> GLVPRGSHMMEILRGSPALSAFRINKLLARFQAANLQVHNIYAEYVHFADLNAPLNDSEQAQLTRLLQYGPALSSHTPAGKLLLVTPRPGTISPWSSKATDIAHNCGLQQVDRLERGVAYYIEASTLTAEQWRQVAAELHDRMMETVFSSLTDAEKLFIHHQPAPVSSVDLLGEGRQALIDANLRLGLALAEDEIDYLQEAFTKLGRNPNDIELYMFAQANSEHCRHKIFNADWIIDGKPQPKSLFKMIKNTFETTPDYVLSAYKDNAAVMEGSAVGRYFADHNTGRYDFHQEPAHILMKVETHNHPTAISPWPGAATGSGGEIRDEGATGRGAKPKAGLVGFSVSNLRIPGFEQPWEEDFGKPERIVTALDIMTEGPLGGAAFNNEFGRPALTGYFRTYEEKVNSHNGEELRGYHKPIMLAGGIGNIRADHVQKGEIVVGAKLIVLGGPAMNIGLGGGAASSMASGQSDADLDFASVQRDNPEMERRCQEVIDRCWQLGDANPILFIHDVGAGGLSNAMPELVSDGGRGGKFELRDILSDEPGMSPLEIWCNESQERYVLAVAADQLPLFDELCKRERAPYAVIGDATEEQHLSLHDNHFDNQPIDLPLDVLLGKTPKMTRDVQTLKAKGDALNRADITIADAVKRVLHLPTVAEKTFLVTIGDRTVTGMVARDQMVGPWQVPVADCAVTTASLDSYYGEAMSIGERAPVALLDFAASARLAVGEALTNIAATQIGDIKRIKLSANWMAAAGHPGEDAGLYDAVKAVGEELCPQLGLTIPVGKDSMSMKTRWQEGNEQREMTSPLSLVISAFARVEDVRHTLTPQLSTEDNALLLIDLGKGHNALGATALAQVYRQLGDKPADVRDVAQLKGFYDAMQALVAARKLLAWHDRSDGGLLVTLAEMAFAGHCGVQVDIAALGDDHLAALFNEELGGVIQVRAEDRDAVEALLAQYGLADCVHYLGQALAGDRFVITANDQTVFSESRTTLRVWWAETTWQMQRLRDNPQCADQEHEAKANDTDPGLNVKLSFDINEDIAAPYIATGARPKVAVLREQGVNSHVEMAAAFHRAGFDAIDVHMSDLLGGRIGLGNFHALVACGGFSYGDVLGAGEGWAKSILFNHRVRDEFETFFHRPQTLALGVCNGCQMMSNLRELIPGSELWPRFVRNHSDRFEARFSLVEVTQSPSLLLQGMVGSQMPIAVSHGEGRVEVRDDAHLAALESKGLVALRYVDNFGKVTETYPANPNGSPNGITAVTTENGRVTIMMPHPERVFRTVANSWHPENWGEDSPWMRIFRNARKQLG

FGAR-AT encoded by the purL gene is a multidomain bi-functional enzyme that catalyzes the fourth step of the purine biosynthesis pathway. The FGAR-AT protein from Salmonella typhimurium (StPurL) has 1295 amino acid residues and is a single chain protein with three major domains. The C-terminal glutaminase domain produces an ammonia molecule that is consumed at the coupled active site present in the formylglycinamidine ribonucleotide (FGAM) synthetase domain where nitrogen is incorporated into an FGAR molecule converting it into FGAM. While the FGAM synthetase domain and glutaminase domain carry out the two enzymatic reactions within this bi-functional enzyme, the function of the N-terminal domain is not clearly understood.

The native crystals of StPurL protein were exposed to xenon gas and it was noticed that crystals derivatized for 5 min or longer at 40 bar, diffracted worse than 4.0 Å resolution. Moreover, solving the structure of StPurL protein crystals (StPurL-Xenon complex) which were pressurized for 4 min did not show any increase in the number of xenon atoms bound as compared to the crystals derivatized for 1 min therefore, 1 min pressurization of xenon was used for further studies. Data sets of the xenon bound structure of StPurL were collected and refined using both native and a mutant version of StPurL R1263A. This mutant was analyzed and was found to be structurally identical to the xenon data set of the native protein (2.65 Å) and diffracted to a higher resolution of 2.18 Å and therefore, used for further analysis. There were no significant changes in the structure on introduction of xenon and the StPurL-Xenon complex was found to be isomorphous to the native structure. However, X-ray crystallographic studies revealed that none of the three internal xenon atoms were trapped in either of the proposed ammonia channels within the protein instead they were bound to select hydrophobic spaces within.>DNVMVSIGPNNTCVPASVFENINWSVCSLATR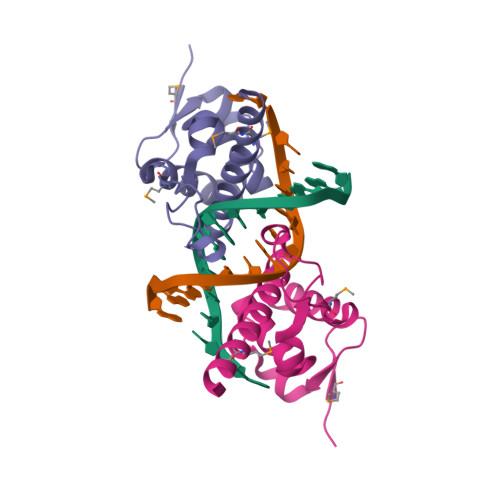KLLVTIFDRETLATHSVTGKPSPAFKDQDKPLKRMLDPGKIQDIIFAVTHKCNASEKEVRNAITTKCADENKMMKIQNVKRRS[2x]> MSLARCERLRGAALRDVLGRAQGVLFDCDGVLWNGERAVPGAPELLERLARAGKAALFVSNNSRRARPELALRFARLGFGGLRAEQLFSSALCAARLLRQRLPGPPDAPGAVFVLGGEGLRAELRAAGLRLAGDPSAGDGAAPRVRAVLVGYDEHFSFAKLREACAHLRDPECLLVATD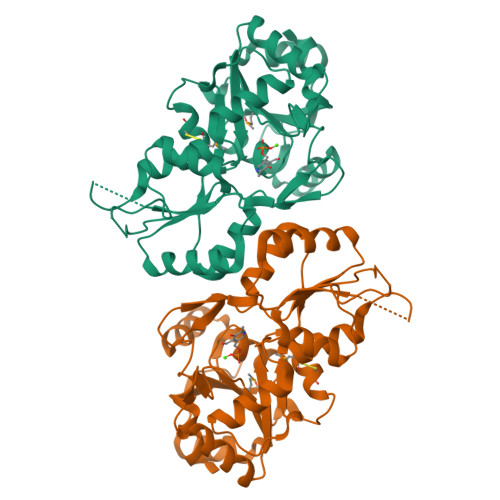RDPWHPLSDGSRTPGTGSLAAAVETASGRQALVVGKPSPYMFECITENFSIDPARTLMVGDRLETDILFGHRCGMTTVLTLTGVSRLEEAQAYLAAGQHDLVPHYYVESIADLTEGLEDEGHHHHHH2,6-DIMETHYL-1-(3-[3-METHYL-5-ISOXAZOLYL]-PROPANYL)-4-[4-METHYL-2H-TETRAZOL-2-YL]-PHENOL 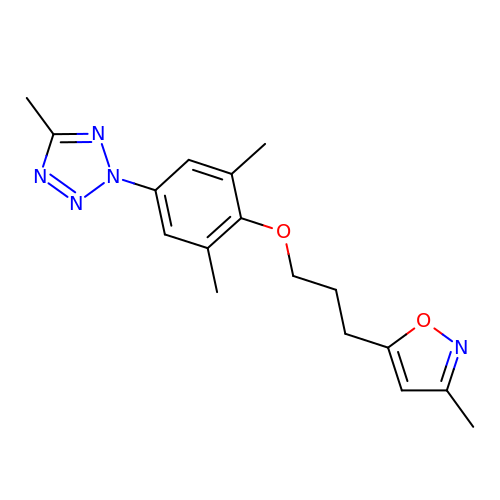| C17 H21 N5 O2 | DRCNRTRGWUYJBH-UHFFFAOYSA-N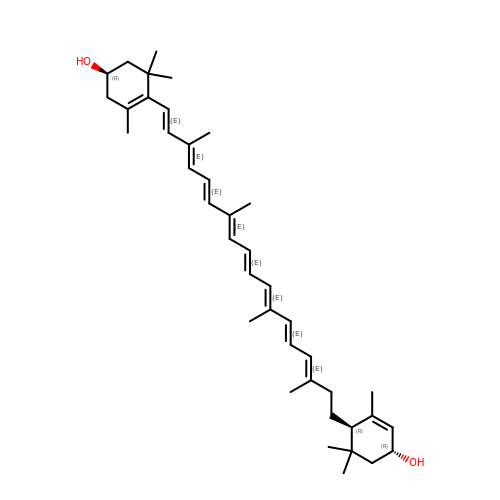(1~{R})-3,5,5-trimethyl-4-[(1~{E},3~{E},5~{E},7~{E},9~{E},11~{E},13~{E},15~{E})-3,7,12,16-tetramethyl-18-[(1~{R},4~{R})-2,6,6-trimethyl-4-oxidanyl-cyclohex-2-en-1-yl]octadeca-1,3,5,7,9,11,13,15-octaenyl]cyclohex-3-en-1-ol | C40 H58 O2 | BVQZFYCQXRWKGU-KTHHOQBFSA-N>[2x]MSGSPAPQGALRQRIVASTPKKTKESKDGAASDAELDKLVKEAAAAKAPAGSERDYKIAFAIITALAFLTRFWGISHPDQVVFDEVHFGKFASYYLQRTYFFDVHPPLGKLLFAFMGWLVGYDGHFHFDNIGDPYVINKVPYVAFRALPAILGSLTVSVVFLIMWESGYSLPACILASGLVLLDNAHIGQTRLILLDATLVFAMACSLLCYIKFYKLRHEPFSRKWWKWLILTGFALSCDISTKYVGLFAFITIGSAVCIDLWDLLNINRPKGALTLPQFGKHFAARAFGLIFMPFMFYLFWFQVHFSILTRSGPGDDFMTPEFQETLSDNIMLANAVTIDYWDTITIKHKETKAYLHSHPDRYPLRYDDGRVSSQGQQVTGYPFNDTNNWWQILPAGPFEEPKLGRHVKHRDLVRLRHVGTDTYLLSHDVASPYYPTNQEFTTVSFNEAYGDRAADTLFEVRIEHGKPGQEFKSISSHFKLIHNPSKVAMWTHPTPLPDWGHRQQEINGNKQIAPSSNVWLVEDIVSLPADHKRREKPERKVKTLPFLRKWFELQRSMFWHNNQLTASHPYASLPYQWPFLLRGVSFWTNSETRQQIYFLGNPVGWWIASSVLAIYVGIVLADQFSLRRGIDALDHRTRSRLYNSTGFFFLAWATHYFPFFVMGRQLFLHHYLPAHLASTLVTGALVEFIFSPEAPEHEIAAQQAKSSSSGKRGGVAMKRHITARERFAGQSLMGSWIATAVILALVAWSWWFFLPLTYGYPGMSVQQVLRRKWLGYDLHFAKLEVLFQGPGSHHHHHHHHHH

Protein O-mannosyltransferases (PMTs) are conserved endoplasmic reticulum membrane-embedded enzymes responsible for the transfer of mannose from dolichol phosphate-mannose (Dol-P-Man) to serine/threonine-rich protein substrates or unfolded proteins. PMTs from three subfamilies form obligate dimers with different substrate specificities and require the concerted action of their transmembrane domains (TMDs) and a luminal MIR domain for catalysis. Here, we present structures, native mass spectrometry, and structure-based mutagenesis of the fungal Pmt4 homodimer. The core fold of the TMDs and MIR domain is conserved with the Pmt1-Pmt2 heterodimer, indicating a shared catalytic mechanism.

Structural analysis by single-particle cryo-electron microscopy (cryo-EM) confirmed ctPmt4 is a homodimer, allowing processing of the data with either no symmetry (C1) or two-fold rotational symmetry (C2) imposed. Within the membrane region, the 3.2 Å C2 map showed the same features as the 3.4 Å C1 map but at higher resolution, and was therefore used to build a two-fold symmetric model for the ctPmt4 transmembrane domains (TMDs). The 11 TMDs of ctPmt4 have a highly similar arrangement to those of scPmt1 and scPmt2, superimposing with a root-mean-square deviation (RMSD) of 1.6 Å and 1.4 Å respectively. Moreover, the ctPmt4 homodimer adopts the same overall morphology within the membrane region as the scPmt1-Pmt2 heterodimer, with a rhombic cavity separating the dimer halves. As in scPmt1-Pmt2, residues at the cytosolic ends of TMD6 (W263 and L266) and TMD8 (R629 and R630) form the major dimer interface, bounding the rhombic cavity on two sides at the cytosolic side of the membrane. However, the luminal ends of TMD9 from each dimer half are tilted further towards each other, resulting in an additional single constriction point at F662 and V663 and a smaller rhombic cavity than for scPmt1-Pmt2. Our cryo-EM reconstructions revealed two single-chain lipid species bound within each membrane domain of the ctPmt4 homodimer, arranged so that the hydrocarbon tails protrude into the central rhombic cavity. The head group of one lipid species is positioned in the luminal membrane leaflet in the active site and was thus modelled as the reaction product Dol-P, as in the scPmt1 structure. The Dol-P phosphate group is also stabilised by the conserved residues H105, K244, R666 and H672, however is retracted 4.7 Å from the acceptor threonine binding site compared to within scPmt1. Strikingly, we found that Dol-P-Man is a good fit for the lipid density in the cytosolic binding pocket, with the phosphate group being stabilised by positively charged residues (R218, R638 and R642) and the mannose group by histidine side chains (H219 and H637).> GSHMASMTGGQQMGRGSGSHMASMTGGQQMGRGSRVGEQSQAGDPGLVSAYGPGLEGGTTGVSSEFIVNTLNAGSGALSVTIDGPSKVQLDCRE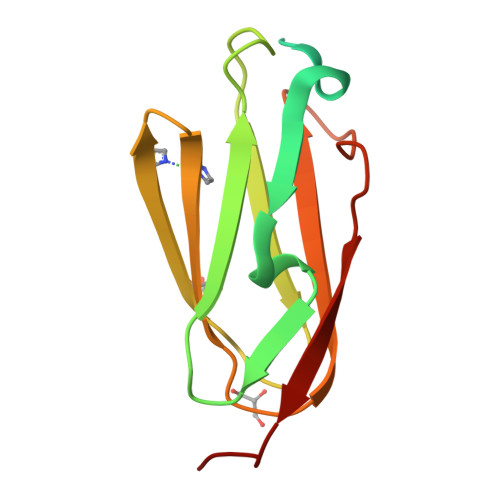CPEGHVVTYTPMAPGNYLIAIKYGGPQHIVGSPFKAKVTGPRLS> VL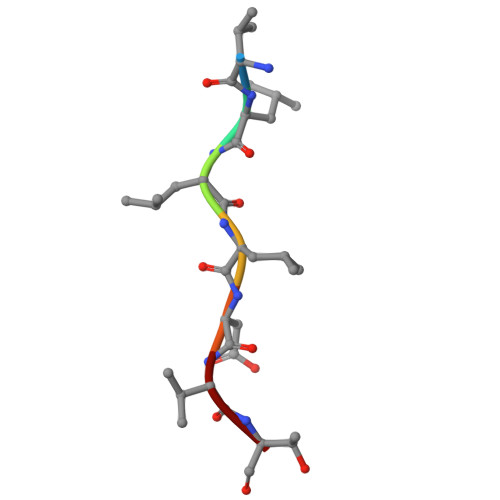LLDVT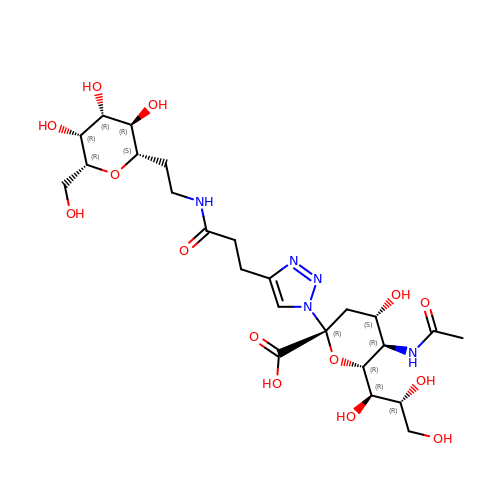(2~{R},4~{S},5~{R},6~{R})-5-acetamido-2-[4-[3-[2-[(2~{S},3~{R},4~{R},5~{R},6~{R})-6-(hydroxymethyl)-3,4,5-tris(oxidanyl)oxan-2-yl]ethylamino]-3-oxidanylidene-propyl]-1,2,3-triazol-1-yl]-4-oxidanyl-6-[(1~{R},2~{R})-1,2,3-tris(oxidanyl)propyl]oxane-2-carboxylic acid | C24 H39 N5 O14 | AWGVVHYVQYXEMI-QRSXIJLLSA-N>GAMDPREVILCKDQDGKIGLRLKSIDNGIFVQLVQANSPASLVGLRFGDQVLQINGENCAGWSSDKAHKVLKQAFGEKITMTIRDRPFERTITMHKDSTGHVGFIFKNGK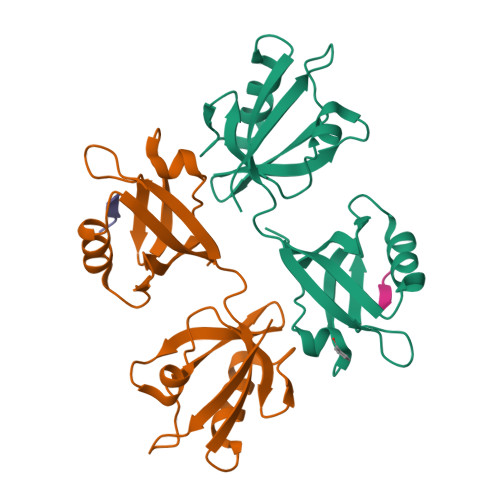ITSIVKDSSAARNGLLTEHNICEINGQNVIGLKDSQIADILSTSGTVVTITIMPAF[2x];>[2x]TNEYKV> LFNSEEDVVKSSPLPTVENQFTPTTAWSTSVGSGIGNF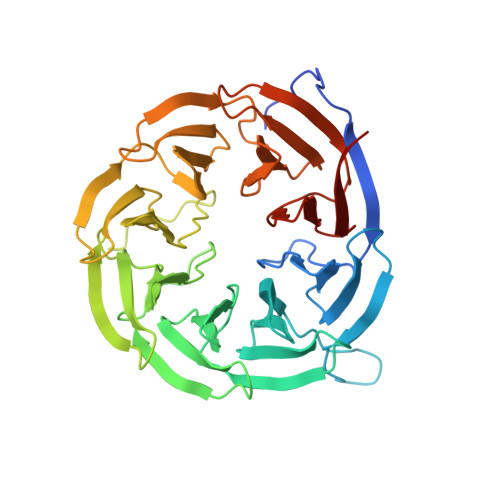YSNLHPALADNVVYAADRAGLVKALNADDGKEIWSVSLAEKDGWFSKEPALLSGGVTVSGGHVYIGSEKAQVYALNTSDGTVAWQTKVAGEALSRPVVSDGLVLIHTSNGQLQALNEADGAVKWTVNLDMPSLSLRGESAPTTAFGAAVVGGDNGRVSAVLMEQGQMIWQQRISQATGSTEIDRLSDVDTTPVVVNGVVFALAYNGNLTALDLRSGQIMWKRELGSVNDFIVDGNRIYLVDQNDRVMALTIDGGVTLWTQSDLLHRLLTSPVLYNGNLVVGDSEGYLHWINVEDGRFVAQQKVDSSGFQTEPVAADGKLLIQAKDGTVYSITRADHHHHHH>MRTQVGIIGAGPAGLLLSHLLYLQGIESIIIENRTREEIEGTIRAGVLEQGTVDLMNQMGVGARMMKEGHFHEGFELRFNGRGHRINVHELTGGKYVTVYAQHEVIKDLVAARLQTGGQIHFNVGDVSLHDVDTSSPKIRFRPNKDGELQEIECDFIAGCDGFRGPSRPAIPQSVRKEYQKVYPFSWLGILVEAPPSAHELIYANHERGFALVSTRSPQIQRLYLQVDAQDHIDNWSDDRIWSELHARLETRDGFKLLEGPIFQKGIVSMRSFVCDPMQHGRLFLAGDAAHIVPPTGAKGLNL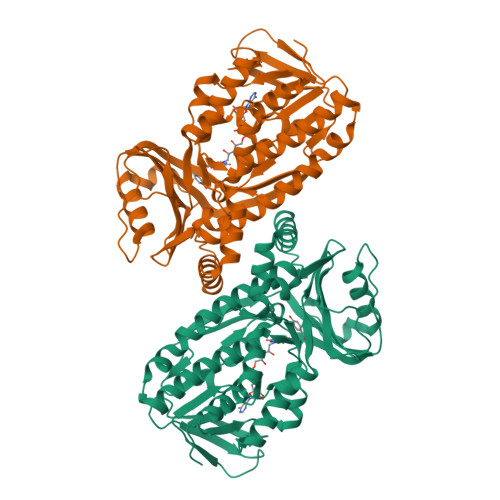AAADVQVLARGLEAYYKAGKMEILNRCTEICLRRIWKAERFSWFMTTMLHRDQGHTPFERGIQLAELDYVTSSRAASTSLAENYIGLPMEFLEHHHHHH[4x]> HSTAETTLDSFFSRAGLVGEIDLPLKGTTNPNGYANWDIDITGYAQMRRKVELFTYMRFDAEFTFVACTPTGEVVPQLLQYMFVPPGAPKPDSRESLAWQTATNPSVFVKLSDPPAQVSVPFMSPASAYQWFYDGYPTFGEHKQEKDLEYGAMPNNMMGTFSVRTVGTSKSKYPLVVRIYMRMKHVRAWIPRPMRNQNYLFKANPNYAGNS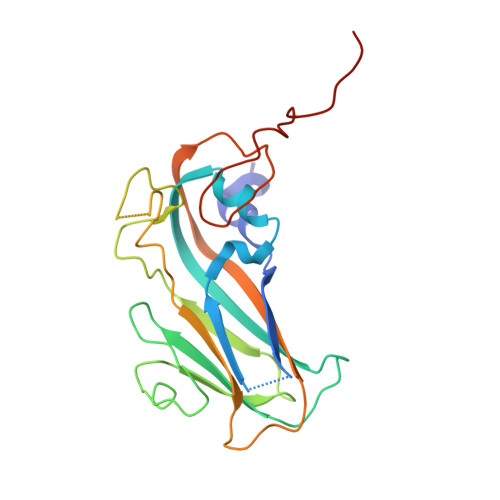IKPTGASRTAITTL> ETQLLKGVLEGCVLDMIGQKERYGYELVQTLREAGFDTIVPGTIYPLLQKLEKNQ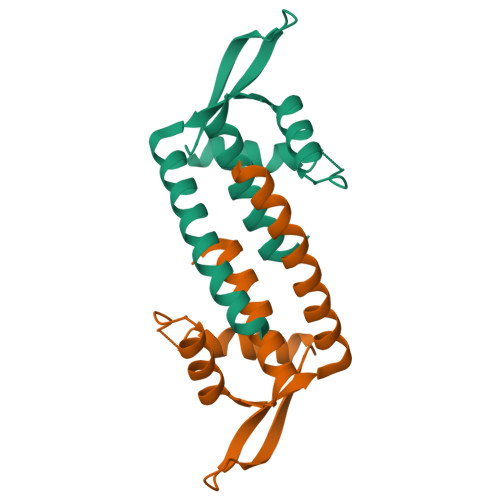WIRGDMRPSPDGPDRKYFSLMKEGEERVSVFWQQWDDLSQKVEGIKN> GGGUACUUAAGCCCACUGAUGAGUCGCUGGGAUGCGAC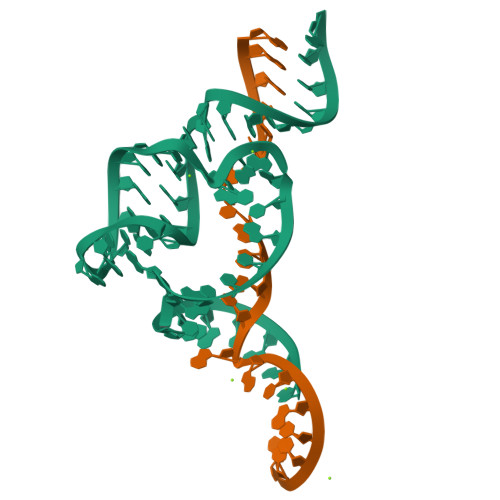GAAACGCCCA;> GGGCGUXUGGGCAGUACCCA>[2x]MAGDPMGNSSTKGSADSKGDKLHVVTTFYPMYEFTKQIVKDKGDVDLLIPSSVEPHDWEPTPKDIANIQDADLFVYNSEYMETWVPSAEKSMGQGHAVFVNASKGIDLMEGSEEEHEEHDHGEHEHSHAMDPHVWLSPVLAQKEVKNITAQIVKQDPDNKEYYEKNSKEYIAKLQDLDKLYRTT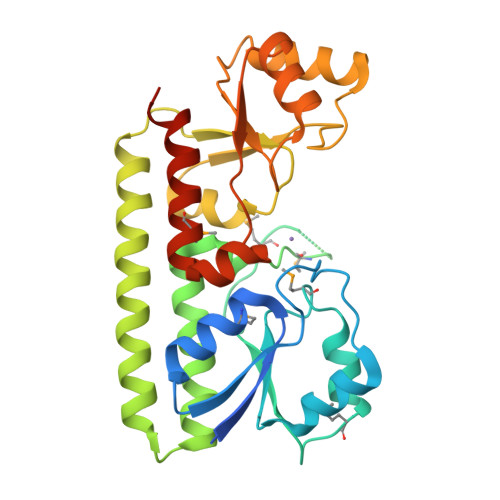AKKAEKKEFITQHTAFGYLAKEYGLKQVPIAGLSPDQEPSAASLAKLKTYAKEHNVKVIYFEEIASSKVADTLASEIGAKTEVLNTLEGLSKEEQDKGLGYIDIMKQNLDALKDSLLVKSLEHHHHHH> LGYGSWEIDPKDLTFLKELGTGQFGVVKYGKWRGQYDVAIKMIKEGSMSEDEFIEEAKVMMNLSHEKLVQLYGVCTKQRPIFIITEYMANGCLLNYLREMRHRFQTQQLLEMCKDVCEAMEYLESKQFLHRDLAARNCLVNDQGVVKVSDFGLSRYVLDDEYT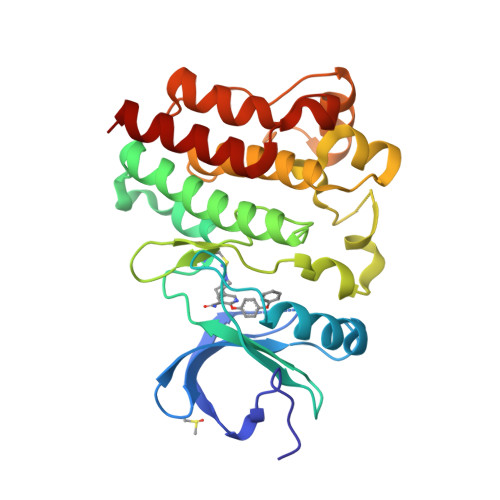SSVGSKFPVRWSPPEVLMYSKFSSKSDIWAFGVLMWEIYSLGKMPYERFTNSETAEHIAQGLRLYRPHLASEKVYTIMYSCWHEKADERPTFKILLSNILDVMDEES>GNQSTSSKGSDTKKEQITVKHQL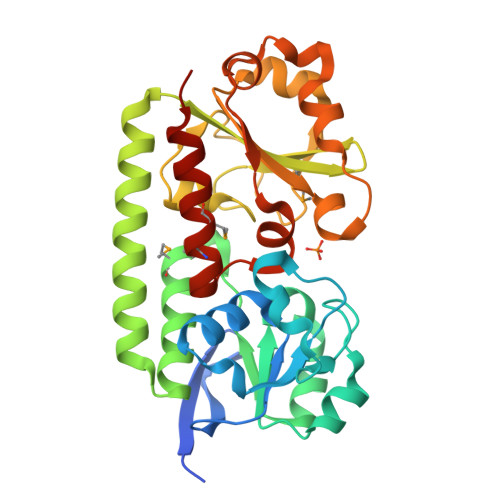DKNGTKVPKNPKKVVVFDFGSLDTLDKLGLDDIVAGLPKQVLPKYLSKFKDDKYADVGSLKEPDFDKVAELDPDLIIISARQSESYKEFSKIAPTIYLGVDTAKYMESFKSDAETIGKIFDKEDKVKDELANIDHSIADVKKTAEKLNKNGLVIMANDGKISAFGPKSRYGLIHDVFGVAPADQNIKASTHGQSVSYEYISKTNPDYLFVIDRGTAIGETSSTKQVVENDYVKNVNAVKNGHVIYLDSATWYLSGGGLESMTQMIKEVKDGLEKENLYFQ[2x]> MHHHHHHMIEWIIRRSVANRFLVLMGALFLSIWGTWTIINTPVDALPDLSDVQVIIKTSYPGQAPQIVENQVTYPLTTTMLSVPGAKTVRGFSQFGDSYVYVIFEDGTDPYWARSRVLEYLNQVQGKLPAGVSAELGPDATGVGWIYEYALVDRSGKHDLADLRSLQDWFLKYELKTIPDVAEVASVGGVVKEYQVVIDPQRLAQYGISLAEVKSALDASNQEAGGSSIELAEAEYMVRASGYLQTLDDFNHIVLKASENGVPVYLRDVAKVQIGPEMRRGIAELNGEGEVAGGVVILRSGKNAREVIAAVKDKLETLKSSLPEGVEIVTTYDRSQLIDRAIDNLSGKLLEEFIVVAVVCALFLWHVRSALVAIISLPLGLCIAFIVMHFQGLNANIMSLGGIAIAVGAMVDAAIVMIENAHKRLEEWQH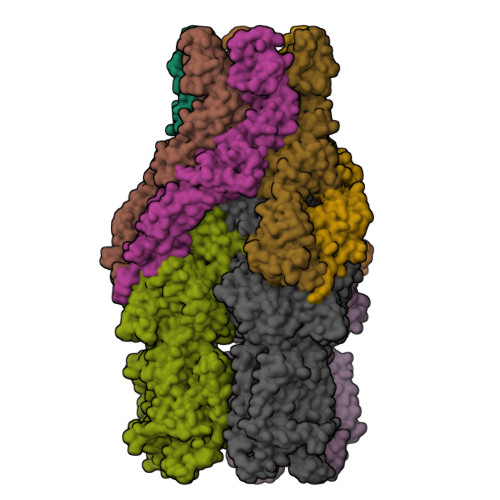QHPDATLDNKTRWQVITDASVEVGPALFISLLIITLSFIPIFTLEGQEGRLFGPLAFTKTYAMAGAALLAIVVIPILMGYWIRGKIPPESSNPLNRFLIRVYHPLLLKVLHWPKTTLLVAALSVLTVLWPLNKVGGEFLPQINEGDLLYMPSTLPGISAAEAASMLQKTDKLIMSVPEVARVFGKTGKAETATDSAPLEMVETTIQLKPQEQWRPGMTMDKIIEELDNTVRLPGLANLWVPPIRNAIDMLSTGIKSPIGIKVSGTVLADIDAMAEQIEEVARTVPGVASALAERLEGGRYINVEINREKAARYGMTVADVQLFVTSAVGGAMVGETVEGIARYPINLRYPQSWRDSPQALRQLPILTPMKQQITLADVADIKVSTGPSMLKTENARPTSWIYIDARDRDMVSVVHDLQKAIAEKVQLKPGTSVAFSGQFELLERANHKLKLMVPMTLMIIFVLLYLAFRRVGEALLIISSVPFALVGGIWLLWWMGFHLSVATGTGFIALAGVAAEFGVVMLMYLRHAIEAVPSLNNPQTFSEQKLDEALYHGAVLRVRPKAMTVAVIIAGLLPILWGTGAGSEVMSRIAAPMIGGMITAPLLSLFIIPAAYKLMWLHRHRVRK;>MKKIALIIGSMIAGGIISAAGFTWVAKAEPPAEKTSTAERKILFWYDPMYPNTRFDKPGKSPFMDMDLVPKYADEESSASGVRIDPTQTQNLGVKTATVTRGPLTFAQSFPANVSYNEYQYAIVQARAAGFIDKVYPLTVGDKVQKGTPLLDLTIPDWVEAQSEYLLLRETGGTATQTEGILERLRLAGMPEADIRRLIATQKIQTRFTLKAPIDGVITAFDLRAGMNIAKDNVVAKIQGMDPVWVTAAIPESIAWLVKDASQFTLTVPARPDKTLTIRKWTLLPGVDAATRTLQLRLEVDNADEALKPGMNAWLQLNTASEPMLLIPSQALIDTGSEQRVITVDADGRFVPKRVAVFQASQGVTALRSGLAEGEKVVSSGLFLIDSEANISGALERMRSESATHAHHHHHHH[2x]> TDLTEEQKETLKKLKLYQKEYYDYESKFEYELFLLRQKYHDLYGPIYDKRREALVGNGEAKIGTPNLPEFWLRALRNNNTVSHVIEDHDEEIL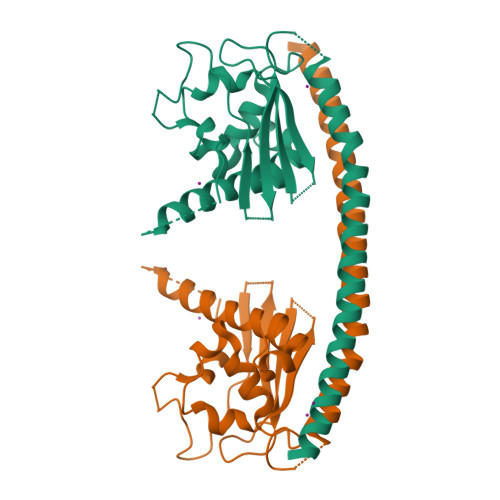VYLNDIRCDYIKKNKEKKEGFILSFYFATNPFFSNSVLTKTYHMKCVDCDNEPVLLHTEATVIDWYDNKNILKKNVVKKQHNKNSREVKTVQQTVNRDSFFHFFTSHKVPNSNVIKQLSKHEVAQLEMIIEGDYEVALTIKERIIPYAVDYYLGII> MSKQRVFIAGHRGMVGSAIRRQLEQRGDVELVLRTRDELNLLDSRAVHDFFASERIDQVYLAAAKVGGIVANNTYPADFIYQNMMIESNIIHAAHQNDVNKLLFLGSSCIYPKLAKQPMAESELLQGTLEPTNEPYAIARIAGIKLCESYNRQYGRDYRSVMPTNLYGPHDNFHPSNSHVIPALLRRF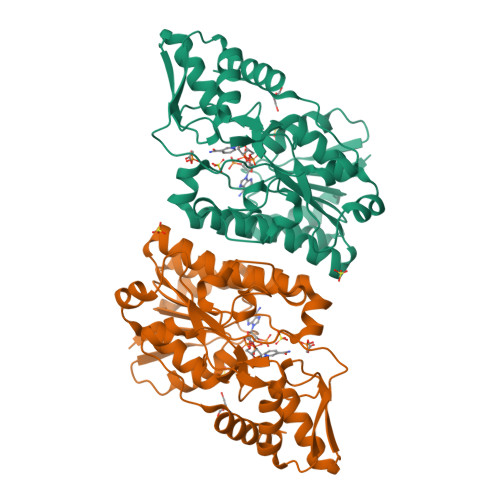HEATAQSAPDVVVWGSGTPMREFLHVDDMAAASIHVMELAHEVWLENTQPMLSHINVGTGVDCTIRELAQTIAKVVGYKGRVVFDASKPDGTPRKLLDVTRLHQLGWYHEISLEAGLASTYQWFLENQDRFRG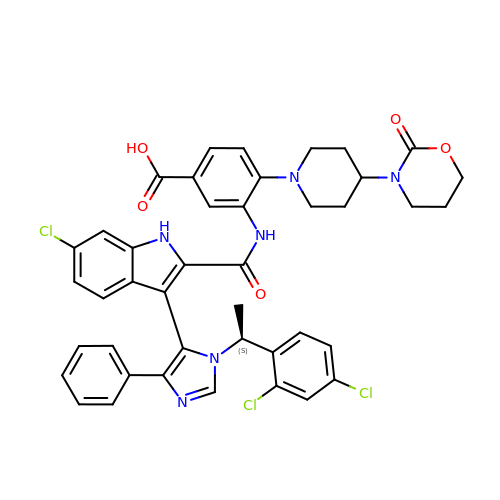3-[[6-chloranyl-3-[3-[(1~{S})-1-(2,4-dichlorophenyl)ethyl]-5-phenyl-imidazol-4-yl]-1~{H}-indol-2-yl]carbonylamino]-4-[4-(2-oxidanylidene-1,3-oxazinan-3-yl)piperidin-1-yl]benzoic acid | C42 H37 Cl3 N6 O5 | GSVXCPWDMIREAJ-DEOSSOPVSA-N>[2x]SNAMSKQFDVVVIGAGPGGYIAAIRAAQLGMSVACIDAWQNGQGGPAPGGTCTNVGCIPSKALLQSSEHYEQANHHFAEHGIEVKGVSLKLDTLIGRKNTVVKQNNDGILYLFKKNKVTYFHGKGAFAGQVDGGWSIKVTGTTDADLVAKHVIVATGSSARELPGLPFDEKNILSNDGALNIGAVPKKLGVIGAGVIGLEMGSVWRRLGAEVTILEAMPEFLAAADQQVAKEALKSFAKQ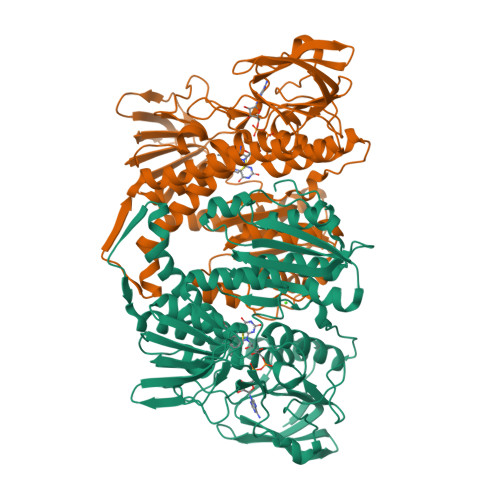GLDIQTGVKIGEIKAAAKSITVPYVDAKGAEQKLVVDKLIVSIGRVPYTGGLNAEAVGLKLDERGFVAVDEDCKTNLPNVWAVGDVVRGPMLAHKAEEEGVAVAERIAGQHGHVNFATVPWVIYTSPEIAWVGKTEQQLKAEGREYKAGSFPFMANGRARALGDTTGFAKVIADAKTDEVLGVHIIGPMASELISEAVTIMEFRGAAEDIARICHAHPTLSEAVKEAALAVDKRTLNF>MTIEKPKISVAFIALGNFCRSPMAEAIFKHEVEKANLENRFNKIDSFGTSNYHVGESPDHRTVSICKQHGVKINHKGKQIKTKHFDEYDYIIGMDESNINN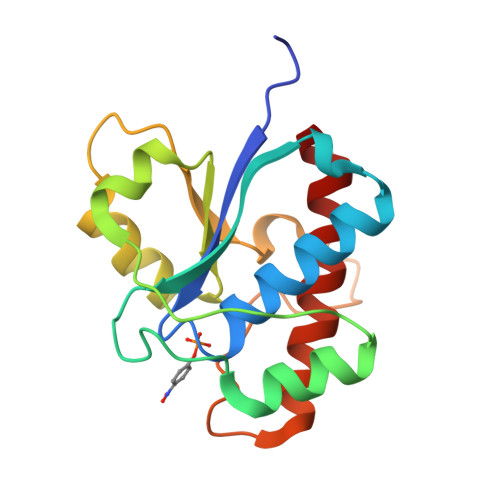LKKIQPEGSKAKVCLFGDWNTNDGTVQTIIEDPWYGDIQDFEYNFKQITYFSKQFLKKEL[2x]We have characterized a new influenza virus from a flat-faced fruit bat (Artibeus planirostris) in the Amazon River basin in northern Peru. While our phylogenetic analysis indicated that the Peruvian bat virus shares common ancestry with recently identified Guatemalan H17N10 bat viruses, their genetic and phylogenetic divergence is such that we propose that their HA and NA genes be designated as new subtypes H18 and N11, respectively. The influenza HA and NA proteins are critical for interaction with the host and determining the subtype of influenza type A viruses. We determined crystal structures of the A/bat/Peru/10 HA and NAL proteins expressed in a baculovirus system.

The extensive sequence divergence of A/bat/Peru/10 NAL from the recently characterized N10 prompted us to determine its X-ray structure in two crystal forms at 2.68 Å and 3.0 Å. The N11 NAL forms a typical “box-shaped” tetramer, containing six four-stranded, antiparallel β-sheets in a propeller-like arrangement. Comparison of the A/bat/Peru/10 NAL monomer with other NA structures reveals surprising similarity despite low sequence identity (29.6%). In addition, a calcium required for stabilization of all known influenza A and B NA active sites is conserved in N11 NAL. Among the eight conserved charged and polar residues that interact with substrate in all other influenza A and B subtypes, only Arg118, Arg224, Glu276 are conserved (N2 numbering) as in N10 NALs. Arg292 and Arg371, critical for sialic acid binding, are replaced in A/bat/Peru/10 NAL by Thr and Lys, respectively. Furthermore, only three of eleven second-shell residues are conserved in N11 NAL (Trp178, Ser179 and Glu425). The N11 NAL active site pocket is much wider than other flu A and B NAs, including 1918 N1, due mainly to 150- and 430-loop movements. The glycerol moiety of a canonical sialic acid, as observed in other flu A and B NA structures, would clash with the N11 NAL active site. N11 NAL catalyzes extremely low levels of sialic acid cleavage as observed for N10 NAL, and similar to H18 HA, N11 NAL exhibited no binding to 610 diverse natural glycans including sialosides in a glycan microarray assay.

>[4x]GSPSRATPLVLGENLCSINGWVPTYRGEGTTGKIPDEQMLTRQNFVSCSDKECRRFFVSMGYGTTTNFADLIVSEQMNVYSVKLGDPPTPDKLKFEAVGWSASSCHDGFQWTVLSVAGDGFVSILYGGIITDTIHPTNGGPLRTQASSCICNDGTCYTIIADGTTYTASSHRLYRLVNGTSAGWKALDTTGFNFEFPTCYYTSGKVKCTGTNLWNDAKRPFLEFDQSFTYTFKEPCLGFLGDTPRGIDTTNYCDKTTTEGEGGIQGFMIEGSNSWIGRIINPGSKKGFEIYKFLGTLFSVQTVGNRNYQLLSNSTIGRSGLYQPAYESRDCQELCFWIEIAATTKAGLSSNDLITFCGTGGSMPDVNWG>MSSLSRELVFLILQFLDEEKFKETVHKLEQESGFFFNMKYFEEKVHAGEWDEVEKYLSGFTKVDDNRYSMKIFFEIRKQKYLEALDRHDRAKAVDILVKDLKVFSTFNEELYKEITQLLTLENFRENEQLSKYGDTKSARSIMLIELKKLIEANPLFREK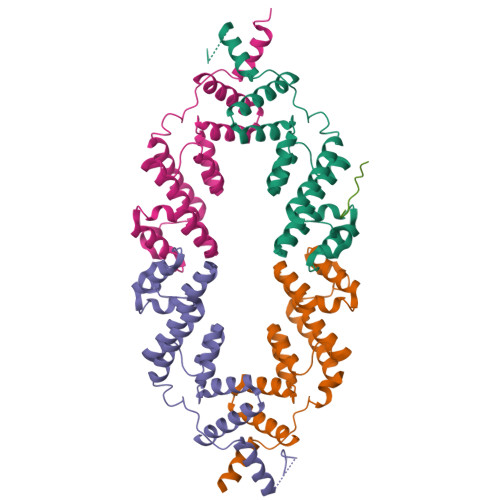LVFPTLKASRLRTLINQSANWQHQLCKNPRPNPDAKTLFTDHTCTPPNG[4x];> DNLIYLDLNLQDWDD>[2x]MHEVEFSHEYWMRHALTLAKRARDEREVPVGAVLVLNNRVIGEGWNRAKGLHDPTAHAEIMALRQGGLVMQNYRLIDATLYST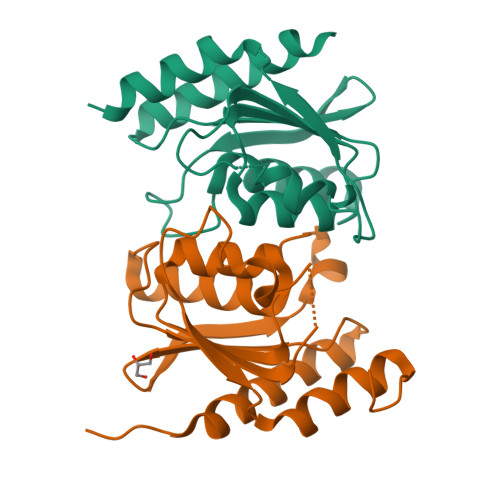FEPCVMCAGAMIHSRIGRVVFGVRNAKTHAAGSLMDVLHHPGMNHRVEITEGILADECAALLCRFFRMPRRVFNAQKKAQSSTD>[2x]GAMAMNGEAICSALPTIPYHKLADLRYLSRGASGTVSSARHADWRVQVAVKHLHIHTPLLDSERKDVLREAEILHKARFSYILPILGICNEPEFL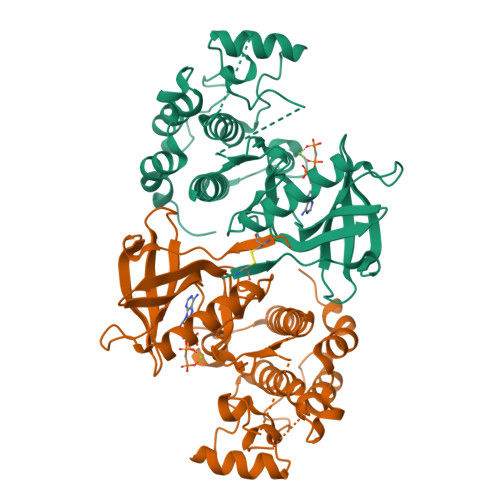GIVTEYMPNGSLNELLHRKTEYPDVAWPLRFRILHEIALGVNYLHNMTPPLLHHDLKTQNILLDNEFHVKIADFGLSKWRMMSLSQSRSSKSAPEGGTIIYMPPENYEPGQKSRASIKHDIYSYAVITWEVLSRKQPFEDVTNPLQIMYSVSQGHRPVINEESLPYDIPHRARMISLIESGWAQNPDERPSFLKCLIELEPVFRTFEEI> GPMLPKGEEGDIIGTFNF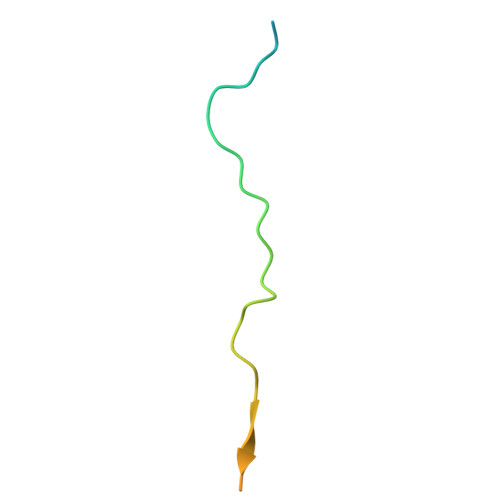SSSDSQPLKIHWVDTPDSSGSNLVPR> SFTSSGMECKNPDSLHVFLVSAPGQGNVTPMLRLAKSLASKGLLVTFSTPESYGKEMRKTNDDISDQPILIGEGSIRFEFLDDEWDENEHKGEGLDAYATHLERVGKQNLPRMFKKHEEEGRPISCIINNPFIPWVPEVAESLGIPSALLWVQSCASFSSYYHFFNDLVSFPTESNLKKDVCLPSMPMLKYDEVPLLLYPIVPLPIISLKNAMLRQQKNLSKTFCVLVDTFQQLEDELIHYLSKLCPIRPIGPLFKISDTSSSNISGDI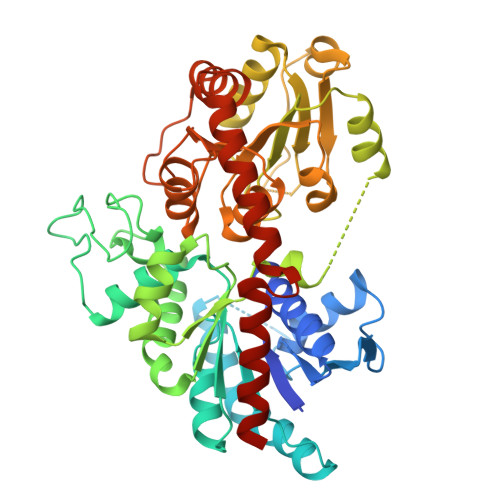RKADDCIEWLDSKSPSSVVYISFGSIVHLKQEQITEIAYALMNINISFLWVMKPPQKDSYDKQHVLPQGFLEKVGEKGKVVKWSPQEQVLSHQSLACFVTHCGWNSSMEALANGIRVVTLPQWGDQVTNAKFLVDVFGVGVRLSRGDLEDRIIPREEIELRLLEVTSGEKATEMKHNALRWKKAAEEAVAKDGSSSKNLQEFVDELNNFRFIT> MTPKTETPVGALIKKFFPGKRFQKNYLKDAGKKLKREGEAAAVEYLSGKQEDHPANFCPPAKVNILAQSRPLSEWPINLVSKGVQEYVYGLTAAEREANGDFGTSRKSLDRWFARTGVPT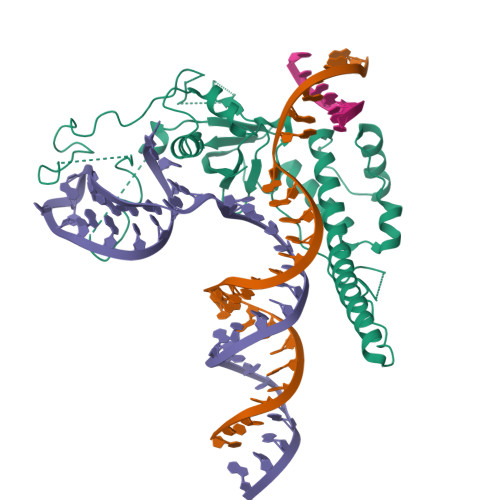HGYTTVQGLNLILRHTFNRYDGVIKKVETRNEKRRSKATRINVSREADGLPPIEAEPEETAFGPDGKLKERPGINPSIYCYQQVSPVPYNPAKHPALPFSGVDPGAPLPLGTPNRLSIPKGQPGYVPEWQRPHLSTKNKRIRKWYARANWRRKPGRKSVLDEAKLKEAALKEAIPIIVTIGKDWIVMDARGLLRAVYWRGIAKPGLSLKELLGFFSGDPVLDPKRGIATFTFKLGAVAV>MAHHHHHHAAARDYTVTAPDGVVLAVQEAGDPEGSPIIFIHGLLGSRLNWSKQLQDPRLQHYRLITYDLRGHGLSGKPAEASSYTDG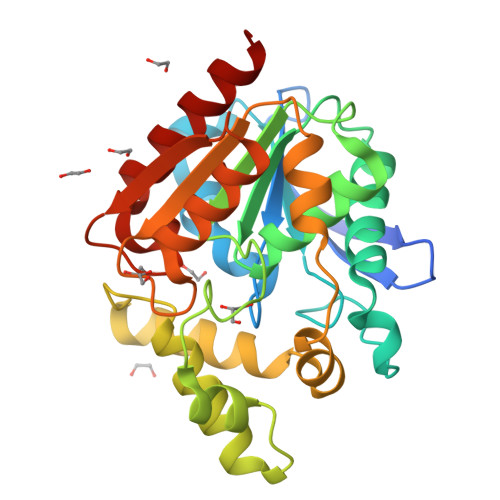RRWADDLAAIIESTHARKPVLVGWSLGGAVISNYLAAYGDKGIAGAVYVDGVIELKPDQIVAHPEVYRDMIASDLQTHLDGERAFLRLCFHRQPDATTFSLLLANAALASWDMQRAVRSMTVEAAKGLSKAEVPLLLLYGAQDALVKAKPSIARAKSLNPRIRSELYADSGHAPFLEEPERFNRDLSDFVRMALSR[4x]>RVMYYG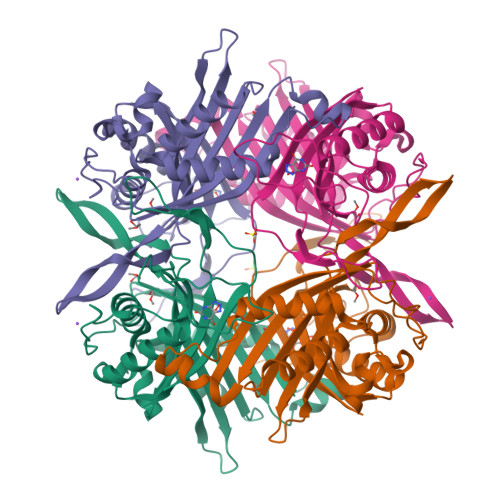KGDVFAYRTYLKPLTGVRTIPESPFSGRDHILFGVNVKISVGGTKLLTSFTKGDNSLVVATDSMKNFIQKHLASYTGTTIEGFLEYVATSFLKKYSHIEKISLIGEEIPFETTFAVKNGNRAASELVFKKSRNEYATAYLNMVRNEDNTLNITEQQSGLAGLQLIKVSGNSFVGFIRDEYTTLPEDSNRPLFVYLNIKWKYKNTEDSFGTNPENYVAAEQIRDIATSVFHETETLSIQHLIYLIGRRILERFPQLQEVYFESQNHTWDKIVEEIPESEGKVYTEPRPPYGFQCFTVTQEDLPHENIL[2x]Methylaminomethyl modification of uridine or 2-thiouridine (mnm5U34 or mnm5s2U34) at the wobble position of tRNAs specific for glutamate, lysine and arginine are observed in Escherichia coli and allow for specific recognition of codons ending in A or G. In the biosynthetic pathway responsible for this post-transcriptional modification, the bifunctional enzyme MnmC catalyzes the conversion of its hypermodified substrate carboxymethylaminomethyl uridine (cmnm5U34) to mnm5U34. MnmC (formally known as YfcK or TrmC) is a bifunctional enzyme responsible for the final two steps of biosynthetic pathway of mnm5s2U in tRNAGlu and tRNALys, and mnm5U in tRNAArg. The C-terminal domain (MnmC1) catalyzes the flavin adenine dinucleotide (FAD)-dependent oxidation of the Cα-N bond in cmnm5U34. The resulting imine intermediate is (presumably) non-enzymatically hydrolyzed to 5-aminomethyl uridine (nm5U34), followed by S-adenosyl L-methionine (SAM)-dependent methylation to yield mnm5U in the N-terminal domain active site (MnmC2).

Here we present the FAD/SAM-bound crystal structures of full-length MnmC from E. coli (ecMnmC) and Y. pestis (ypMnmC), and an FAD-bound crystal structure of ypMnmC. In the FAD- and FAD/SAM-bound ypMnmC structures, of the 689 residues, the first 28 N-terminal residues, 183–184, 451, and 602–609 are not represented by electron density. The ~30 disordered N-terminal residues in the ypMnmC structures are near SAM binding site; however, this conformational flexibility does not appear to affect SAM binding, as the ligand was fully occupied in crystals of ypMnmC which had been soaked in mother liquor containing 5 mM SAM. Our structures show that ecMnmC and ypMnmC bind SAM in an almost identical manner. Although the overall architecture of the binding pocket is highly similar, a few additional residues are found within hydrogen bonding distance from SAM in ypMnmC; e.g., Thr-69, Asn-72, Asp-156, and Asp-178, which interact via their side chains, and Leu-71, Asn-72 and Val-157 via backbone amide group. SAM-bound structures of both ecMnmC and ypMnmC show that Asp-178 is the only charged residue near SAM, except for Glu-101, which anchors the ribosyl moiety through multiple hydrogen bonds with its side chain. The distance between Cϵ of SAM and Oδ of the Asp-178 side chain is 4.1 Å in ecMnmC and 3.6 Å in ypMnmC. In addition, the side chains of Phe-24 and Phe-180 contact the nucleoside segment of SAM, shielding it from bulk solvent in the ecMnmC structure, although Phe-24 is not visible due to disorder in ypMnmC structure. The binding mode of SAM within the MnmC2 domain was examined by soaking pre-existing crystals, which did not elicit any significant structural alteration of the MnmC2 domain or reorganization of the MnmC1/MnmC2 interface. YpMnmC and ecMnmC share 61% overall sequence identity and exhibit similar structural organization with an RMSD of 1.1 Å calculated over 626 Cαs.

> MNQRPIQTATLSWNEQGTPVSEQFGDIYFSNEDGLEETHHVFLKGNGFPARFASHPQQSCIFAETGFGTGLNFLTLWRDFALFRQQSPNATLRRLHYISFEKYPLHVADLASAHARWPELASFAEQLRAQWPLPLAGCHRILLADGAITLDLWFGDVNTLLPTLDDSLNNQVDAWFLDGFAPAKNPDMWNEQLFNAMARMTRPGGTFSTFTAAGFVRRGLQQAGFNVTKVKGFGQKREMLTGTLPQQIHAPTAPWYHRPAATRCDDIAIIGGGIVSALTALALQRRGAVVTLYCADAQPAQGASGNRQGALYPLLNGKNDALETFFTSAFTFARRQYDQLLEQGIAFDHQWCGVSQLAFDDKSRGKIEKMLHTQWPVEFAEAMSREQLSELAGLDCAHDGIHYPAGGWLCPSDLTHALMMLAQQNGMTCHYQHELQRLKRIDSQWQLTFGQSQAAKHHATVILATGHRLPEWEQTHHLPLSAVRGQVSHIPTTPVLSQLQQVLCYDGYLTPVNPANQHHCIGASYQRGDIATDFRLTEQQENRERLLRCLPQVSWPQQVDVSDNQARCGVRCAIRDHLPMVGAVPDYAATLAQYQDLSRRIQHGGESEVNDIAVAPVWPELFMVGGLGSRGLCSAPLVAEILAAQMFGEPLPLDAKTLAALNPNRFWIRKLLKGRPVQTRSPATQESSR Our work utilizes biotin–streptavidin (Sav) technology to develop artificial metalloproteins (ArMs) that mimic the active sites of natural copper metalloenzymes. Our group develops artificial metalloproteins (ArMs) using biotin–streptavidin (Sav) technology to mimic natural metalloenzyme active sites to characterize otherwise elusive intermediates and study the effects of the secondary coordination sphere on metal ion(s) reactivity. This approach leverages the strong binding affinity between biotinylated metal complexes and the Sav host to confine synthetic metal cofactors within a protein scaffold. By engineering ArMs with aromatic residues within their secondary coordination spheres, we systematically investigate the influence of these residues on Cu reactivity and oxidant activation. Our results demonstrate how the inclusion of aromatic residues within the secondary coordination sphere influences the structure and reactivity of copper ArMs.

Based on the observations that positioning of the tyrosine is important for promoting activity, we reasoned that oxidation of phenylalanine residues might also be achievable while maintaining the cofactor geometry and orientation. We were able to successfully prepare and characterize the S112F variant or [CuII-biot-et-dpa⊂2XM-S112F-K121Y-Sav], where the molecular structure determined by X-ray diffraction reveals that F112 can maintain support of the N49 coordination to the Cu cofactor (Fig. S24†). However, after several attempts, in crystallo reactivity studies of 4 with H2O2 were inconclusive due to heterogeneity and disorder within the crystals. It is possible that the increased disorder of the F112 structures upon H2O2 exposure is caused by the lack of a stabilizing H-bond, exhibited by Y112 in 1, with the backbone carbonyl of A121. Nevertheless, both the intact protein mass spectrum and enzymatic digest analysis reveal peaks corresponding to specific oxidation of 4 upon peroxide-treatment. Additionally, the rotameric change and coordination of N49 in 1 and 4 also suggested its potential role in reactivity. When the location is appropriate, such as in the case of S112Y and S112F, steric constraints shift Cu center towards N49, allowing amide coordination and then S112Y and S112F are readily oxidized upon exposure to H2O2.

> MASMTGGQQMGRDEAGITGTWYNQLGSTFIVTAGADGALTGTYESAVGNAESRYVLTGRYDSAPATDGSGTALGWTVAWKNNYRNAHSATTWSGQYVGGAQARINTQWLLTFGTTEANAWASTLVGHDTFTKVKPSAASIDAAKKAGVNNGNPLDAVQQ1-(4-iodophenyl)-3-[2-(4-sulfamoylphenyl)ethyl]thiourea | C15 H16 I N3 O2 S2 | 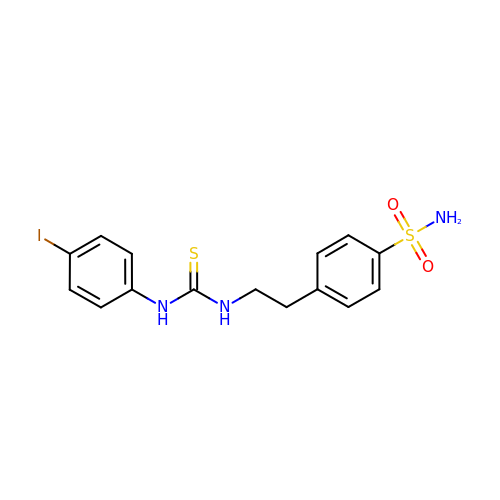JUSYUNJKOKPYPO-UHFFFAOYSA-N>[2x]LKLTESNRSPRTTNTTDLSGKVAVVTGAAAGLGRAEALGLARLGATVVVNDVASALDASDVVDEIGAAAADAGAKAVAVAGDISQRATADELLASAVGLGGLDIVVNNAGITRDRMLFNMSDEEWDAVIAVHLRGHFLLTRNAAAYWRDKAKDAEGGSVFGRLVNTSSEAGLVGPVGQANYAAAKAGITALTLSAARALGR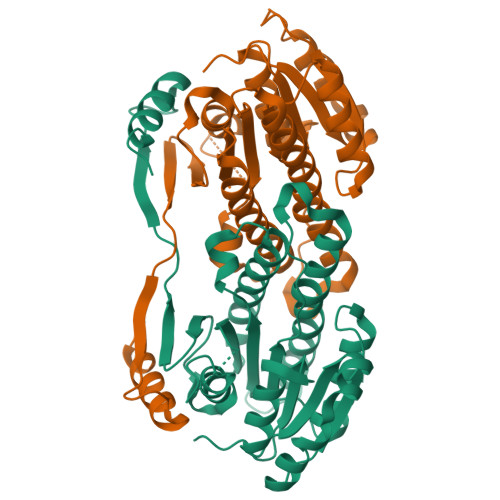YGVCANVICPRARTAMTADVFGAAPDVEAGQIDPLSPQHVVSLVQFLASPAAAEVNGQVFIVYGPQVTLVSPPHMERRFSADGTSWDPTELTATLRDYFAGRDPEQSFSATDLMRQ> MRGSHHHHHHGSMVKQIESKTAFQEALDAAGDKLVVVDFSATWCGPCKMIKPFFHSLSEKYSNVIFLEVDVDDCQDVASECEVKCMPT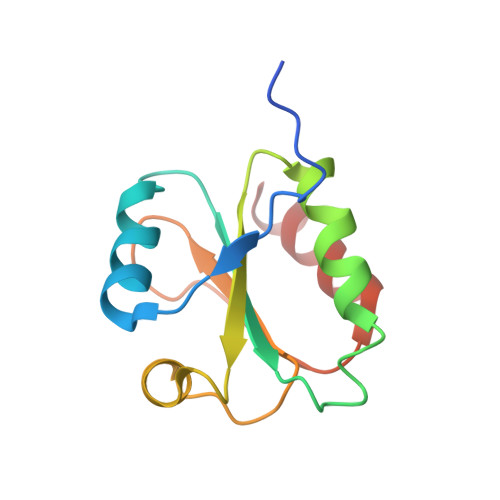FQFFKKGQKVGEFSGANKEKLEATINELV>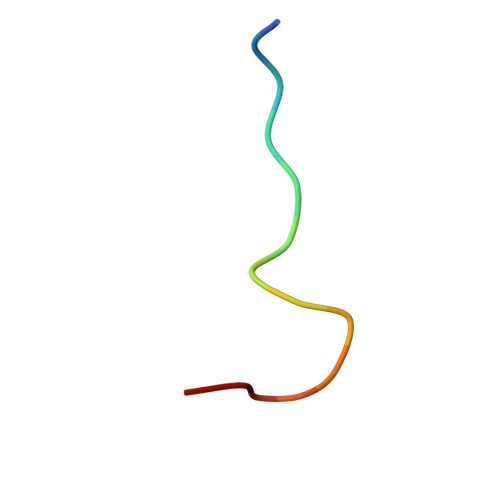 DLAVGPPSLNYPGY Dehydroquinate dehydratase (DHQD) catalyzes the conversion of 3-dehydroquinic acid (DHQ) into 3-dehydroshikimic acid in the mid stage of the shikimate pathway, which is essential for the biosynthesis of aromatic amino acids and folates. Here, we report two the crystal structures of type II DHQD (CgDHQD) derived from Corynebacterium glutamicum, which is a widely used industrial platform organism. The enzyme forms a homododecamer consisting of four trimers with three interfacial active sites. Our analysis revealed that the monomer is composed of repetitive α/β domains, forming a flavodoxin fold with central parallel β sheets arranged in a specific order.

We determined the structures for CgDHQDWT with the citrate at a resolution of 1.80Å and CgDHQDR19A with DHQ complexed forms at a resolution of 2.00 Å, respectively. The asymmetric unit of the citrate- and DHQ-bound structures contained four and six molecules, respectively, highly homologous with alpha carbon, with root mean square deviation values within 0.2. The citrate ion exerts a weak inhibitory effect on DHQD, which is enzyme-dependent. The CgDHQD structure in complex with the citrate ion exhibits two different binding modes of the molecule. The citrate ions bound in two CgDHQD chains in the asymmetric unit are stabilized by the side chains of R19, Y24, N75, H81, H101, S103, and R112 and the main chains of S103 and I102. The citrate-binding mode is similar in that the stabilization of 3-carboxyl and 3-hydroxyl groups resembles that of 1-carboxyl and 1-hydroxyl groups of DHQ, as observed in the structure of Helicobacter pylori DHQD. However, the other binding mode of citrate in the other chains in the asymmetric unit is uncommon, wherein the molecule is accommodated in the active site with a half-opened lid loop. In this mode, the 3-hydroxyl group of the citrate molecule is rotated by almost 180° compared to that in the general binding mode, and the molecule does not interact with the residues R19, Y24, H81, and R112, which are essential in the general binding mode. This unique binding mode illustrates the possibility of various interactions for inhibitor binding that do not mimic perfectly fitted substrate binding. We identified the DHQ-binding site of CgDHQD and observed an unusual binding mode of citrate inhibitor in the site with a half-opened lid loop.

>[4x]MPGKILLLNGPNLNMLGKREPDIYGHDTLEDVVALATAEAAKHGLEVEALQSNHEGELIDALHNARGTHIGCVINPGGLTHTSVALLDAVKASELPTVEVHISNPHAREEFRHHSYISLAAVSVIAGAGIQGYRFAVDILANLKKLEHHHHHH> GSMISGIRVNDNCVTEFNNMKIRKTCGWIIFVIQNCEIIIH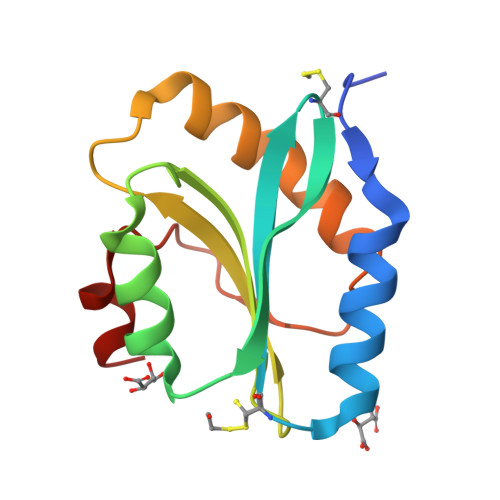SKGASTTLTELVQSIDKNNEIQCAYVVFDAVSKIHFFMYARESSNSRDRMTYASSKQAILKKIEGVNVLTSVIESAQDVADLK> MKHHHHHHMKQNSPLDEENLTQENQDRGTHVDRGLASANVDFAFSLYKQLVLKAPDKNVIFSPLSISTALAFLSLGAHNTTLTEILKGLKFNLTETSEAEIHQSFQHLLRTLNQSSDELQLSMGNAMFVKEQLSLLDRFTEDAKRLYGSEAFATDFQDSAAAKK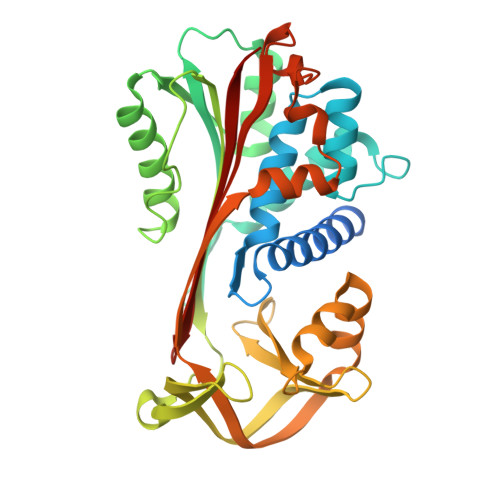LINDYVKNGTRGKITDLIKDLDSQTMMVLVNYIFFKAKFEMPFDPQDTHQSRFYLSKKKYVMVPMMSLHHLTIPYFRDEELSCTVVQLNYTGNASALFILPDQDKMEEVEAMLSQETLARFFDSLEFREIGELYLPKFSISRDYNLNDILLQLGIEEAFTSKADLSGITGARNLAVSQVVHKAVLDVFEEGTEASAATALEVLFQ> GAMAQEIELKFIVNHSAVEALRDHLNTLGGEHHDPVQLLNIYYETPDNWLRGHDMGLRIRGENGRYEMTMKVAGRVTGGL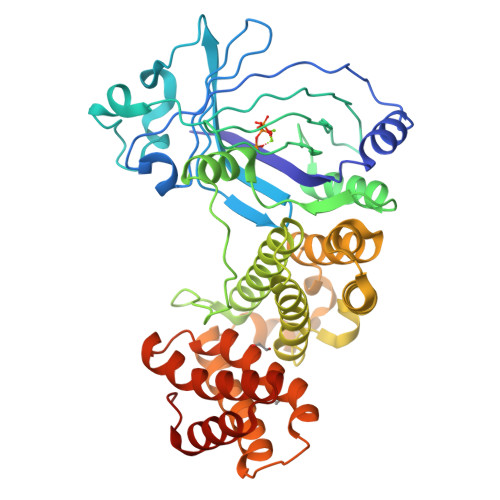HQRPEYNVALSEPTLDLAQLPTEVWPNGELPADLASRVQPLFSTDFYREKWLVAVDDSRIEIALDQGEVKAGEFAEPICELELELLSGDTRAVLKLANQLVSQTGLRQGSLSKAARGYHLAQGNPAREIKPTTILHVAAKADVEQGLEAAFELALAQWQYHEELWVRGNDAAKEQVLAAIGLVRHALMLFGGIVPRKASTHLRDLLTQCEATIASAVSAVTAVYSTETAMAKLALTEWLVSKAWQPFLDAKAQGKISDSFKRFADIHLSRHAAELKSVFCQPLGDRYHDQLPRLTRDIDSILLLAGYYDPVVAQAWLENWQGLRHAIATGQRIEIEHFRNEANNQEPFWLHSGKR> GSTPHLVNLNEDPLMSECLLYHIKDGVTRVGQVDMDIKLTGQFIREQHCLFRSIPQPDGEVVVTLEPCEGAET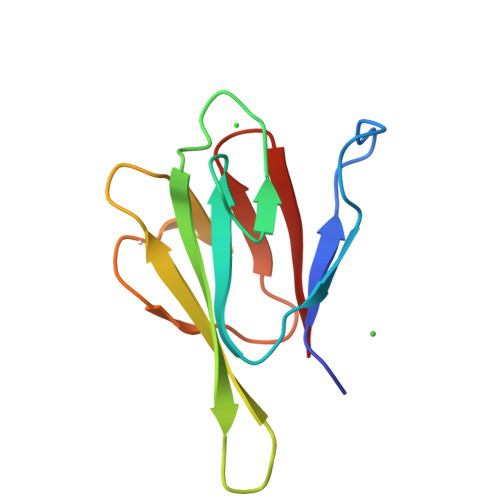YVNGKLVTEPLVLKSGNRIVMGKNHVFRFNH> ENALLRYLLDK;> KPEPTDEEWELIKTVTEAHVATNAQGSHWKQKRKFLPEDIGQAPIVNAPEGGKVDLEAFSHFTKIITPAITRVVDFAKKLPMFCELPCEDQIILLKGCCMEIMSLRAAVRYDPESETLTLNGEMAVTRGQLKNGGLGVVSDAIFDLGMSLSSFNLDDTEVALLQAVLLMSSDRPGLACVERIEKYQDSFLLAFEHYINYRKHHVTHFWPKLLMKVTDLRMIGACHASRFLHMKVECPTELFPPLFLEVFE

The thyroid hormone receptors (THRs) are nuclear hormone receptors regulated by endogenous thyroid hormones, including the inactive prohormone thyroxine (T4) and the bioactive hormone 3,3′,5-triiodothyronine (T3), which are critical for development regulation and metabolic homeostasis. As ligand-regulated nuclear receptors, THRs have a structurally conserved LBD that allows the binding of distinct ligands (Burris et al., 2013). Following the ligand binding, the function of THRs is mediated through the selective recruitment or release of specific coregulators, like the family of steroid receptor coactivators (SRCs) (Li et al., 2003, Jin and Li, 2010, Savkur and Burris, 2004), as a heterodimeric complex with retinoid X receptor (RXR) (Putcha et al., 2012, Kojetin et al., 2015, Mangelsdorf and Evans, 1995). Although the defects in any of the processes in thyroid hormone transport and synthesis can all contribute to RTH, in most cases the disorder involves defective thyroid hormone receptors, resulting in reduced T3 binding and disruptive thyroid hormone signaling.

Surprisingly, roxadustat (FG-4592), a first-in-class oral hypoxia-inducible factor prolyl hydroxylase (HIF-PH) inhibitor and recently approved drug for the treatment of anemia, was revealed as a positive THRs activator. With a molecular scaffold distinct from native thyroid hormones, roxadustat strongly promoted the interaction of both THRα and THRβ with various coactivator LXXLL motifs from the family of steroid receptor coactivators (SRC1, SRC2, and SRC3) with EC50s of about 25 and 15 nM, respectively (see Transparent Methods and Figures S2, 1A, and 1B), suggesting an agonist nature of the ligand. To determine the molecular basis of the binding selectivity of roxadustat to THRβ, we solved the crystal structures of THRβ LBD complexed with roxadustat. The structure reveals that the roxadustat-bound THRβ adopts a canonical active conformation in a three-layer helical sandwich arrangement that resembles most agonist-bound nuclear receptor structures, in agreement with the agonist activity of roxadustat on THRs by both AlphaScreen and reporter assays. The existence of roxadustat was apparent from the highly revealing electron density map shown in Figure 2B, whose interaction with THRβ was stabilized by a combination of hydrogen bonds and hydrophobic interactions. Notably, structural alignment of THRβ-bound roxadustat with various THR ligands available at PDB revealed that roxadustat shares a conserved carboxyl head group for all the THR ligands (Nascimento et al., 2006, Sandler et al., 2004, Huber et al., 2003, Dow et al., 2003, Ye et al., 2003, Borngraeber et al., 2003, Hangeland et al., 2004, Bleicher et al., 2008, Koehler et al., 2006). Despite that roxadustat overall aligns well with T3, a unique structural feature of roxadustat different from T3 is its extended hydrophobic phenyl group, suggesting that a larger hydrophobic cavity is needed for the effective ligand binding.>[2x]MGSDKIHHHHHHENLYFQGMIQEIASILVQPGREADFEAGVAQARPLFM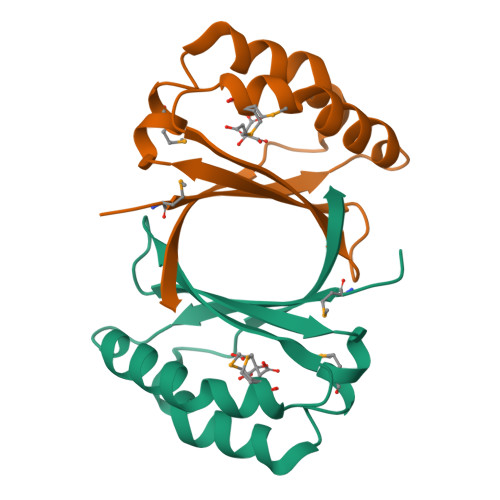RARGCHGVALHRSIEAPQRYTLVVDWETVDNHMVDFRQSADFQEWRKLVGECFAEPPQVHHEQKVL>[4x]TATYSGNPFVGVTPWANAYYASEVSSLAIPSLTGAMATAAAAVAKVPSFMWLDTLDKTPLMEQTLADIRTANKNGGN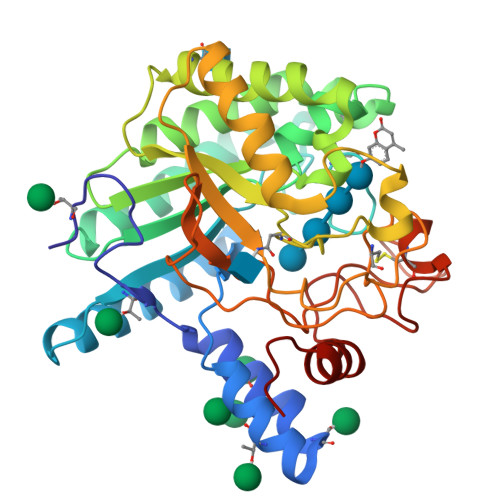YAGQFVVYDLPDRDCAALASNGEYSIADGGVAKYKNYIDTIRQIVVEYSDIRTLLVIEPASLANLVTNLGTPKCANAQSAYLECINYAVTQLNLPNVAMYLDAGHAGWLGWPANQDPAAQLFANVYKNASSPRALRGLATNVANYNGWNITSPPSYTQGNAVYNEKLYIHAIGPLLANHGWSNAFFITDQGRSGKQPTGQQQWGDWCNVIGTGFGIRPSANTGDSLLDSFVWVKPGGECDGTSDSSAPRFDSHCALPDALQPAPQAGAWFQAYFVQLLTNANPSFL>MAKVLVLYYSMYGHIETMARAVAEGASKVDGAEVVVKRVPETMPPQLFEKAGGKTQTAPVATPQELADYDAIIFGTPTRFGNMSGQMRTFLDQTGGLWASGALYGKLASVFSSTGTGGGQEQTITSTWTTLAHHGMVIVPIGYAAQELFDVSQVRGGTPYGATTIAGGDGSRQPSQEELSIARYQG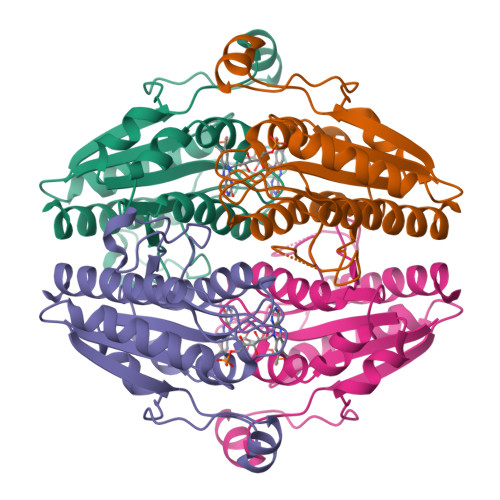EYVAGLAVKLNG[2x]> MHHHHHHHHMRGVRRILPFLGPAVIASIAYMDPGNFATNIEGGARYGYSLLWVILAANLMAMVIQNLSANLGIA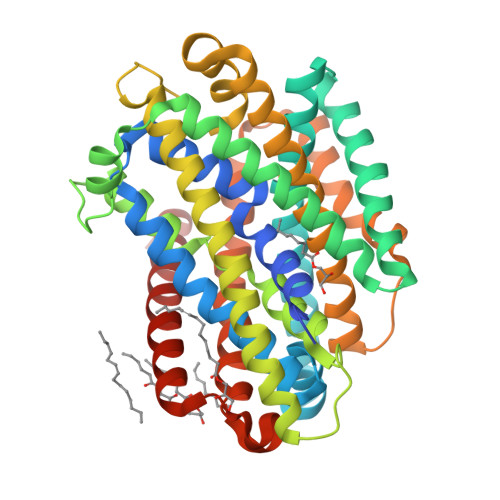SGRNLPELIRERWPRPLVWFYWIQAELVAMATDLAEFLGAALAIQLLTGLPMFWGAVVTGVVTFWLLNLQKRGTRPLELAVGAFVLMIGVAYLVQVVLARPDLAAVGAGFVPRLQGPGSAYLAVWIIGATVMPHVIYLHSALTQGRIQTDTTEEKRRLVRLNRVDVIAAMGLAGLINMSMLAVAAATFHGKNVENAGDLTTAYQTLTPLLGPAASVLFAVALLASGLSSSAVGTMAGDVIMQGFMGFHIPLWLRRLITMLPAFIVILLGMDPSSVLILSQVILCFGVPFALVPLLLFTARRDVMGALVTRRSFTVIGWVIAVIIIALNGYLLWELLGG> MIDFLKQLPHLEPYGNPFYFIYLGIALLPIFIGLFFKKRFAIYECLVSITFIVLALTGTHASQILALLFYIVWQIIWVYSYKRYRSQRDNKWVFYLHSFLVVLPLILVKVEPTINGTQSLLNFLGISYLTFRAVGMIIEMRDGVLKEFTLGEFLRFMLFMPTFTSGPIDRFKRFNEDYQSIPNRDELLNMLEQAVKYIMLGFLYKFVLAQIFGSMLLPPLKAQALSQGGIFNLPTLGVMYVYGFDLFFDFAGYSMFALAVSNLMGIKSPINFDKPFISRDMKEFWNRWHMSLSFWFRDFVFMRLVIVLMRNKVFKNRNTTSNVAYIINMMVMGFWHGITWYYIAYGIFHGIGLVINDAWLRKKKTINKDRKKAGLKPLPENKWTKALGIFITFNTVML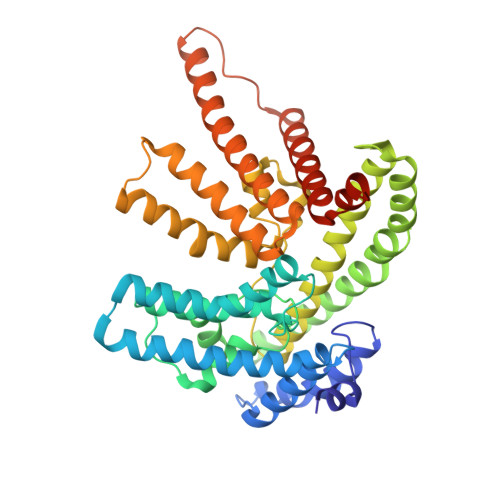SFLIFSGFLNDLWFTKKLEHHHHHHHH>[3x]MVQISEVRGNTRDHRTAAHTHIKGLGLNSSGIAEKQAAGFVGQCAAREACGVVVDLIKAHKMAGRGVLLAGGPGTGKTALALAISQELGTKIPFCPITGSEIYSTEVKKTEVLMENFRRAIGLRVRETKDVYEGEVTEMTPEEAENPLGGYGKTISTLLIGLKSARGQKKLRLDPSIYEAIQKERVQVGDVIYIETNTGACKRVGRSDAYATEFDLEAEEYVPIPKGEVHKKKEIVQDVTLHDLDVANARPQGGQDIISMMGQLMKPKMTEITDKLRMEINKVVQKYINQGVAELIPGVLFIDEAHMLDIECFTYLNKALESPIAPIVVLASNRGIATIRGADDLKAAHGIPPDFLQRLLIIPTHPYEPDEIRRIVRIRAQTEGVQLTDAAVDRVAEHGVRISLRYCLQLLAPASILARVNGRTQVDVQDIAEAEELFLDARRSANILTSTGESGGLHGFIS;>[3x]MAAPLVTSVTETKELRGLNLIAAHSHIRGLGVDADTLEPRPSSQGLVGQEKARKAAAVVLEMIKQGKIAGRAVLIAGPPSTGKTAIAMGMAQSLGQDVPFTTLAASEIFSLEMSKTEALTQAFRKSIGVRIKEESEIMEGEVVEIQIDRSVTGGAKQGKLTIKTTDMEAIYDMGSKMIDAMTKERVMAGDIISIDKSSGKITKLGRSYARSRDYDAMGVDTKFLQCPEGELQKRKEVVHTVSLHEIDVINSRTQGFLALFSGDTGEIRSEIRDQINTKVAEWKEEGKAEIVPGVLFIDEVHMLDIECFSYINRALESDLAPIVIMASNRGVSRIRGTDYKSPHGLPLDFLDRVVIINTHPYTPDELRQILSIRAQEEEVDLTPDALALLTKIGQEAGLRYASNLITTSQLIAAKRRAKQVGVEDVQRSFKLFYDPARSVRFVQESEKRLIGNDGVVDFSYQGAAEAAAPTLPAAAPVDPVGGEKMDMS;> MTDSYATKASNLKKTAILASKEAKRWQLRTNKGTKDLQARAKRVMRDMMGFWKRNEREERDLRKAAERLELENARKEEADREAARQRRKLNFLISQTELYSHFISKKIKTHEVERSTDHPDVATDEKDKIPEPTLNINVPEPTGPIAPKVTDFNSLDFDNEDESALQAAAMANAQNAIAEAQKKAREFNKDETKLDEDGEMNFQHPELTEFEVAQPKLLNCQLKEYQLKGLNWLVNLYEQGINGILADEMGLGKTVQSISVMAYLAERYDIWGPFLVVAPASTLHNWQQEVSKFVPDFKVLPYWGTAADRKVLRKFWDRKHTTYKKDSPFHVMITSYQLVVSDVAYFQKMKWQYMILDEAQAIKSSQSSRWKCLLGFHCRNRLLLTGTPIQNNMQELWALLHFIMPSLFDSHDEFSEWFSKDIESHAQSNTKLNEDQLKRLHMILKPFMLRRVKKHVQKELGDKIEIDVFCELSYRQRAMYQSLRNQISIMDLIEKATVGDNEDSATLMNLVMQFRKVCNHPDLFERADTSSPFFCGHFAETGSFLREGTNVALGYSTRSLVEYRLPRLIWCDGGRLDKPGPGNLVAGF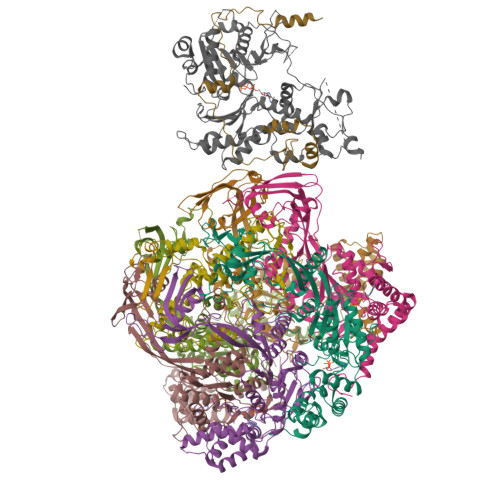RSKYLNHMMNIWTPENIRSSLEGIENFTWLRFVDTSLQEAYRASHTDVFARAVDLASKQNRLGHMQIVYDEPEDKKWTPVHALFQICERENPKAVAEITTEGVLRDLMNIARVKYRELGLCRLEKAARPRASAPPIEVVCDSRSAVIERENIMFHPAMRKALFGPTPSEIKEASFGPRPVTLYPPRALLPAPDHDKQRFTNITVPSMARFVTDSGKLAKLDELLRELKEGGHRVLLYFQMTRMIDLMEEYLTYRNYKYCRLDGSTKLEDRRDTVADFQTRPEIFIFLLSTRAGGLGINLTTADTVIFYDSDWNPTIDSQAMDRAHRLGQTKQVTVYRLITRGTIEERIRKRALQKEEVQRVVITGTGSVDFSGRRPPENRNRDIAMWLADDEQAEMIERREKELIESGEYDKIMQQRRKGGKRKRGAANGDTVPSLEDMYHEGEGHFDDNKGSGAATPVDADSLGRGGKRKKAGGSKKAKTTKQRLAIADGEIDDGEIDIDYKDDDDKGTDYKDDDDK;> MSTRPRRHAAQRASQAITDLADRDRESDHSHGPISSRMSSFNSSSRSRLPGKGIASVSRSEAGGASDPEHIHLTVKLPSSKLRQATSSSGIKKAGSVGSSSSSSGGGKAAVKRARGGKRSRVLESSEEEEEENEVEVLGDEDEEEEEEEDEIEVREGEGYDEDEEDVEDEDEEMQDLGEEDADGEDDEMDVDAEGEEDADGDVNMDAGVVGARATTVRAVPPAIKVTKPPKESPSNGKAATASKANDNAVPVKRPAPDSDDESLSSLESEPEEEVNVAGGEDAEGEDDDAEGEVDAEGEEEEEEEEIEVADEDAEGEDVEQDEDEDEEEEDDDDEMISRAQTPDMSRLTARQRARLGEASGEYLKLSDEVQSKKHFTAEELSMRRAEMARRRRNLSEKRNEEIKMETVNKLLKKQAPRTTRRAAQAAAAAEEAEEAAKQPKRPDPMMIRWVNNKMGSVVAVPEELLGTHAGVVFGAGPGKGLPAGKMVEEV;> MSNPDAQSAQAAHQALVEQLDLHSIHKTFRNPNWRPNQRRNKTIKAILGESQRKEASSTSAVATPRADDNGGGSGADTPANNDNNDGLSTSGTSTPANGNGSGAGTPASNGQPNLAQASRSLQKLVLEKSLASAQAPDKKAANGFASSAPTATYTNIESAPSLAPMKHYCDVTGLPAPYLDPKTRLRYHNKEIFAMIRNLPQGMGEQFLEARGAHTVLK;> MAPSAVAEPPPIPQRDEPWKRLPPPTVYPVKEARFEKYIPPQLDGRERALAQPPGQVAIVIDNGSHSVRAGWNFEDKPRLAIPPIMSKYRDRKMGKTFSFAGSDCYADTTARSHIRNAFEAGTGIVSNWDVMEHVLDYVFVKLGMNECDGAIDMPIVMTEAVANLPYSRKSMSEIIFECYGAPSLVYGIDSLFSFRHNQGQTGLVVSSSYSATHVIPVYNRKALLSQAIRLNWGGWHMAEYMLKLLKLKYYTGFPGKLNSSQTEHMVRDFCYVSLDYDRELAGYLDWTGLEDRERIVQYPYTEEVVVQKTEEELARIAERKKESGRRLQEQAAKMRLERLMKKEQELEYYKDIQRRMQGESKKEIKRLLDEAELKDEAALERVIRDLERSIKRARQKDLGEPEEEEVPDFSLLDVPDDQLDEAGLRQKRQQRLLKSNWEARQRAKAEKEAEKARLAEEARLDEERRKNDLEGWLEEKRQLRLAKLNQLKERERLKADLGNRKSLASQIRMKNIANLASDNPTGSGSRKRRRGGAGADQDDDFGADDADWGVYRSVAIGANKGDDSDDEEGEEDLEAAIRSLENDLLRYDKTFSYDMTLDAQRDWSKSLLHAFRYGPRPFDPSSQAETHRVHLNVERIRVPEVLFQPAAIAGVDQAGLVEIAGDILCQRLPSLPGIQDAPDAFLRDVFLTGGNTLFQNFDERLRQGLMALLPVGAPLRVRRAQDAILDAWRGAAGWACTEEAKAAWITREEYLEKGGEYIKEHDLGNAFA>[4x]S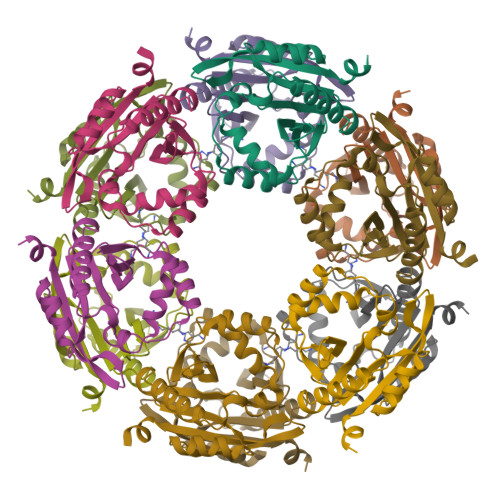NAMKLRALEYSDLLFVHELNNEYSIMSYWFEEPYESLTELQHLFDKHLLDESERRFIVEDENQVVGIVELVEINYIHRNCEIQIIIKPEFSGKGYAKFAFEKAIIYAFNILNMHKIYLYVDADNKKAIHIYESQGFKTEGLLKEQFYTKGKYKDAYFMSLLKSEYIL>MRFTLKTTAIVSAAALLAGFGPPPRAAELPPGRLATTEDYFAQQAKQAVTPDVMAQLAYMNYIDFISPFYSRGCSFEAWELKHTPQRVIKYSIAFYAYGLASVALIDPKLRALAGHDLDIAVSKMKCKRVWGDWEEDGFGTDPIEKENIMYKGHLNLMYGLYQLVTGSRRYEAEHAHLTRIIHDEIAANPFAGIVCEPDNYFVQCNSVAYLSLWVYDRLHGTDYRAATRAWLDFIQKDLIDPERGAFYLS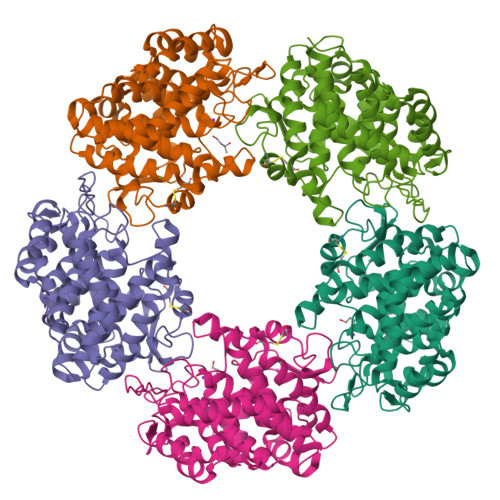YHPESGAVKPWISAYTTAWTLAMVHGMDPAFSERYYPRFKQTFVEVYDEGRKARVRETAGTDDADGGVGLASAFTLLLAREMGDQQLFDQLLNHLEPPAKPSIVSASLRYEHPGSLLFDELLFLAKVHAGFGALLRMPPPAAKLAGK[5x]> MTSSSGVDNEISLDSPMPIFNESSTLKPIRVAGVVTTGTDHIDPSVLQAYLDDTIMKSITLGQLVKNADVLNKRLCQHHIALNAKQSFHFQGNTYISDEKETHDVVPLMEVVSQLDILPPKTFTAKTGTNFGNDNDAEAYLQFEKLIDKKYLKLPTRVNLEILRGTKIHSSFLFNSYSSLSPQSILNLKVFSQFYNWNTNKGLDIGQRGARLSLRYEPLFLHKLLHNPHSNESPTLFH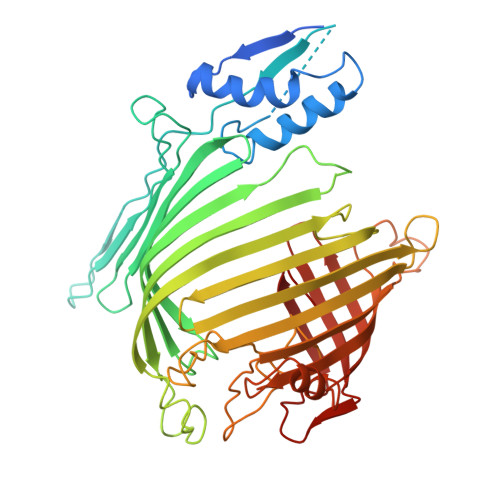EWFLETCWRSTKICSQGTSAPYMYSGTMLSQAGDQLRTILGHTFVLDKRDHIMCPTKGSMLKWSNELSPGKHLKTQLELNSVKSWMNDDFITFSTTIKTGYLKNLSSQQSLPVHICDKFQSGGPSDIRGFQTFGLGPRDLYDAVGGDAFVSYGLSVFSRLPWKKVEKSNFRLHWFFNGGKLVNHDNTSLGNCIGQLSKEHSTSTGIGLVLRHPMARFELNFTLPITAHENDLIRKGFQFGLGLAFL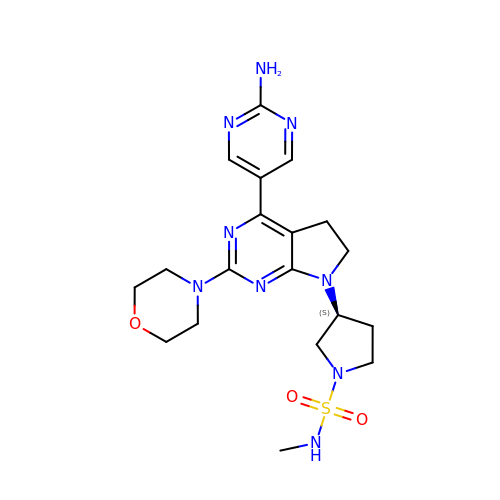(3S)-3-[4-(2-aminopyrimidin-5-yl)-2-(morpholin-4-yl)-5,6-dihydro-7H-pyrrolo[2,3-d]pyrimidin-7-yl]-N-methylpyrrolidine-1-sulfonamide | C19 H27 N9 O3 S | GDUURIYHJNAYDO-AWEZNQCLSA-N>GMSSSGIEIAKPFVTATTNVLSTMAGIQPIPGQP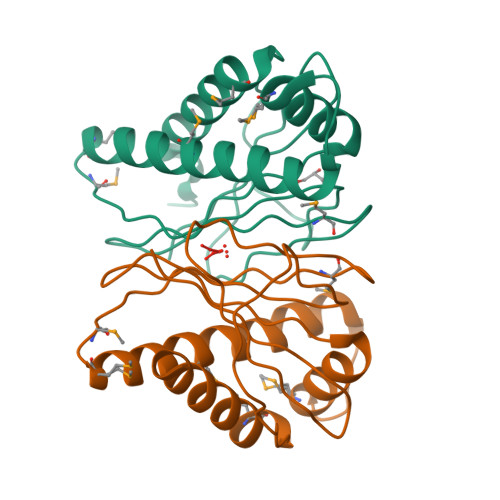YVKKNNVAKGDVSAVVGITGHKNGSISVTFTKQCAIAVVKAMLGDDIQDIIQDTKDAVGEVTNMISGQARAALSEMGMTFQGATPSVIMGDGHTISHVTKSPVIAIPFKTNHGEFTVEFCLE[2x]> AMENKIEVNNKDEMNRWFEEFKKGNGLVDTFTNSYSFCESIPNLDRFVFQMASATDDAQKDSIYASALVEATKFCAPIYECAWVSSTGIVKKGLEWFEKNAGTIKSWDESYTELKVDVPKIEQLTGYQQAALKWRKDIGFRVNANTAALSNKVLAEYKVPGEIVMSVKEMLSDMIRRRNLILNRGGDENPRGPVSHEHVDWCREFVKGKYIMAFNPPWGDINKSGRSGIALVATGLAKLAETEGKGIFDEAKKTVEALNGYLDKHKDEVDRASADSMITNLLKHIAKAQELYKNSSALRAQSAQIDTAFSSYYWLYKAGVTPETFPTVSQFLFELGKQPRGTKKMKKALLSTPMKWGKKLYELFADDSFQQNRIYMHPAVLTAGRISEMGVCFGTIPVANPDDAAQGSGHTKSILNLRTNTE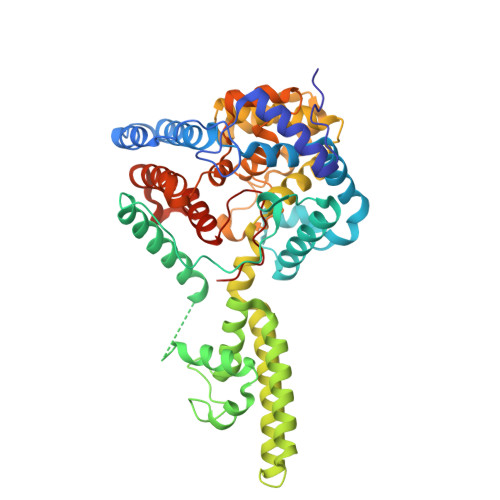TNNPCAKTIVKLFEVQKTGFNIQDMDIVASEHLLHQSLVGKQSPFQNAYNVKGNATSANII>MTQNSQAMTSHAMTGDFVLPELEDVRAEAATVDTRAVLALAEGEEPAESRAAVALALWEDRSIG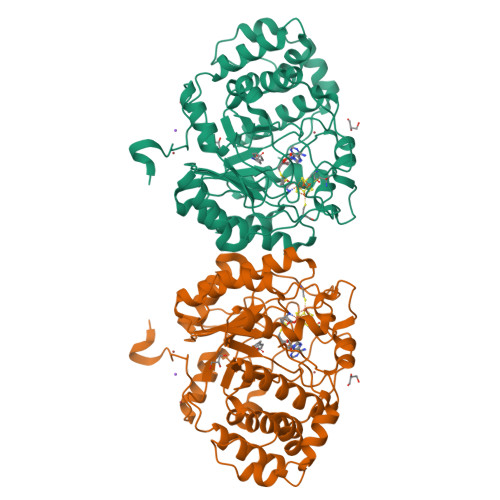TAELQAAAEARCGARRPRLHTFVPLYTTNYCDSECKMCSMRKGNHRLDRKFSGRKEITEQLEILYHHEGVRGVGFLTGEYEDKHTRLASAFRIGWAIRTALDLGFERVYFNIGSMEQDEIDVLGEWIGREDPVTMCVFQESYDRETYRRFMGKTSVGVPKADFDRRVVSFDRWLDAGYRYVNPGVLVGLHDDLSAELVSLVAHGDHLRSRGATADLSVPRMRPAMKSRDTTRVGDDDYLRLMSVVAFTCPEQRLVLTTREPQEFQDVALGLAGVISPGSPDVAPYRAGCEARNDEKSSQFLVADLRRPRHILGRIEASGTPVDHFVNPAGEASRAV[2x]> TVES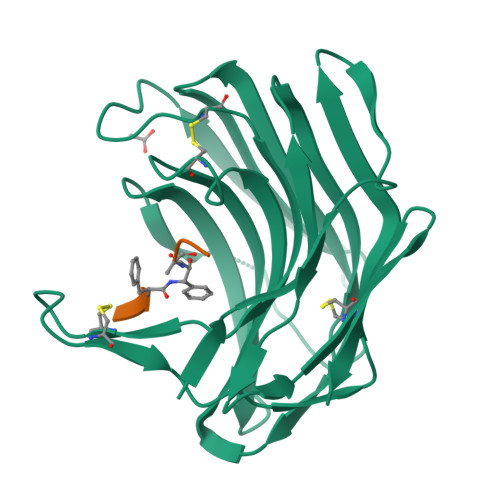NWGGAILIGSDFDTVSATANVPSASGGSSAAGTAWVGIDGDTCQTAILQTGFDWYGDGTYDAWYEWYPEVSDDFSGITISEGDSIQMSVTATSDTSGSATLENLTTGQKVSKSFSNESSGSLCRTNAEFIIEDFEECNSNGSDCEFVPFASFSPAVEFTDCSVTSDGESVSLDDAQITQVIINNQDVTDCSVSGTTVSCSYV>ALALDTPLPTPSGWTTMGDVAVGDHLLGPDGEPTRVVADTDVMLGRPCYVVEFSDGTAIVADAQHQWPTEHGVRITANLRAGMHTVVSASGGRGGTALLAPAVQITAVRRRPSVPVRCVEVDNPEHLYLAGPGMVPTHN[3x]

Inteins are intervening polypeptide domains that conditionally catalyze their own excision from flanking exteins, rendering a functional host protein. DnaB, a hexameric helicase that denatures double-stranded DNA by ATP hydrolysis, is essential for DNA replication and thus for survival. In M. smegmatis, DnaBi1 lacks a homing endonuclease (HEN) domain and is located in the ATP-binding P-loop, and its sequence and insertion site are evolutionarily conserved in some mycobacteria, including M. leprae. DnaBi1 utilizes a noncanonical mechanism known as class 3 splicing where an internal cysteine (C118), rather than a cysteine or serine at the first position of the intein, performs the initial nucleophilic attack.

We therefore set out to solve the structure of DnaBi1 bound to zinc to understand the precise nature of DnaBi1 splicing inhibition. The DnaBi1-zinc complex crystallized in monoclinic space group P1 21 1. The asymmetric unit consisted of five zinc ions and three DnaBi1 molecules (referred to as A, B, and C). The zinc-bound structure of DnaBi1 is nearly identical to that of the apo DnaBi1 (root mean square [RMS] deviation of 0.065). Among the five zinc ions, one is bound at the molecular interface between molecule A and molecule B within the three DnaBi1 molecules in the asymmetric unit. Three other zinc ions bind to each DnaBi1 molecule in identical positions. These three zinc ions are coordinated by sulfur on C118, peptide backbone atoms (N and O) of V119, and the hydroxyl group (OH) of Y128 of each DnaBi1. Additionally, V119 and Y128 are found within a conserved splicing block of DnaBi1. Consistent with our SDR results obtained using our KD154 sensor in M. smegmatis, as well as our findings using the MIG reporter, zinc inhibition of DnaBi1 splicing was found to occur through direct binding to the initiating nucleophile for protein splicing.> MDRLTPLLSGWLDKLSPQGNYVFQRRFVQFNGRSLMYFGSDKDPFPKGVIPLTAIEMTRSSKDNKFQVITGQRVFVFRTESEAQRDMWCSTLQSCLKEQRLLGLEHHHHHH

Arap3, a dual GTPase-activating protein (GAP) for the small GTPases Arf6 and RhoA, plays key roles in regulating a wide range of biological processes, including cancer cell invasion and metastasis. Arap3 structurally consists of an N-terminal sterile alpha motif (SAM) domain, two catalytic GAP domains, ArfGAP and RhoGAP, a Ras-associating (RA) domain and five pleckstrin homology (PH) domains. PI(3,4,5)P3 binding is essential for Arap3 function, which drives recruitment of Arap3 to the plasma membrane to facilitate interaction with its GTPase substrates. Arap3-PH1 domain adopts a canonical PH domain fold, which consists of a seven-stranded β-barrel that is capped at one end by a long C-terminal α-helix.

To understand how Arap3-PH1 domain recognizes PI(3,4,5)P3, we determined the crystal structures of unliganded and diC4-PI(3,4,5)P3-bound Arap3-PH1 domain, which refined to 2.1 and 3.3Å resolution, respectively. The other end of the β-barrel is open and features three loops (β1/β2, β3/β4 and β6/β7), which are hypervariable in both length and sequence in presently known PH domain structures. However, sequence analyses show that Arap3-PH1 contains a KXnQXR motif in the β1-β2 region, which is identical to the canonical KXn(K/R)XR motif in PIPs binding-PH domains, except for the substitution of (K/R) residue by Gln (Q306) in Arap3-PH1. The overall structures of Arap3-PH1 in free and in complex are almost identical, with an overall Ca RMSD of 0.85 Å. However, a significant structural change upon diC4-PI(3,4,5)P3 binding is observed in the region of β1/β2 loop (S298-V304), which exhibits an outward movement, with a Ca RMSD of 1.52 Å. However, our structure data suggested that residues preceding L290, including P288 and L289, interact with the PH1 domain core and may contribute to the structural integrity and stability of the protein.> MSLGTSEQSEIREIVAGSAPARFARGWHCLGLAKDFKDGKPHSVHAFGTKLVVWADSNDEIRILDAYCRHMGGDLSQGTVKGDEIACPFHDWRWGGNGRCKNIPYARRVPPIAKTRAWHTLDQDGLLFVWHDPQGNPPPADVTIPRIAGATSDEWTDWVWYTTEVDTNCREIIDNIVDMAHFFYVHYSFPVYFKNVFEGHVASQFMRGQAREDTRPHANGQPKMIGSRSDASYFGPSFMIDDLVYEYEGYDVESVLINCHYPVSQDKFVLMY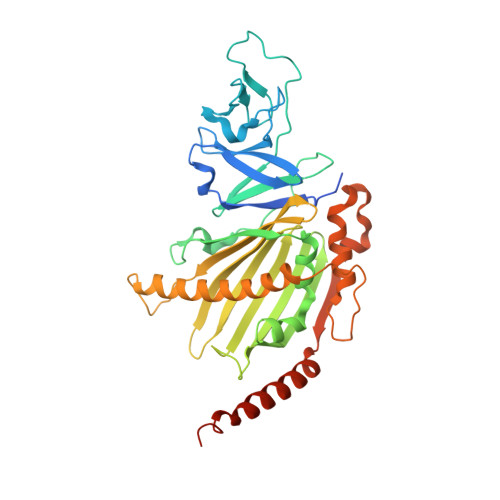GMIVKKSDRLEGEKALQTAQQFGNFIAKGFEQDIEIWRNKTRIDNPLLCEEDGPVYQLRRWYEQFYVDVEDVAPEMTDRFEFEMDTTRPVAAWMKEVEANIARKAALDTETRSAPEQSTTAG> ASTSKTIEELQQEMEDLDADTTITVVQRETQKARIREQIETLRAQQMVRPSEAQLQPDVTPTQIVTFEPPRVTGFGALWIPRQQRNYMTTAYIEKIKAYVPHSNLIESGLASEAQLTSWIENTCRDYQVSMDVFMTTVLPAWIVNCIINGTSQERTNEHTWRAVIMANMEDQEVLYYPIKPIIVNAQPTLRQVMRHFGEQAVAQYMNSLQAGKPFTVKGAVTAGYANVQDAWLGIDFLRDTMQLTTKQMEVKHQIIAANVTRRKIRVFALAAPGDGDELDTERHVVDDVARGRHSLRGAQLD

Sweet potato feathery mottle virus (SPFMV) and Sweet potato mild mottle virus (SPMMV) are members of the genera Potyvirus and Ipomovirus, family Potyviridae, sharing Ipomoea batatas as common host, but transmitted, respectively, by aphids and whiteflies. A common feature for all potyvirids is the structure of virions as non-enveloped, flexible rod-shaped particles, composed of multiple copies of a unique coat protein (CP) helically arranged around the RNA genome. Here we report the generation of virus-like particles (VLPs) by transient expression of the CPs of SPFMV and SPMMV in the presence of a replicating RNA in Nicotiana benthamiana. Analysis of the purified VLPs by cryo-electron microscopy, gave structures with resolutions of 2.6 and 3.0 Å, respectively, showing a similar left-handed helical arrangement of 8.8 CP subunits per turn with the C-terminus at the inner surface and a binding pocket for the encapsidated ssRNA.

The structures of SPFMV and SPMMV were determined using single particle cryoEM with helical symmetry, at resolutions of 2.6 Å (SPFMV) and 3.0 Å (SPMMV). Each subunit is separated by helical rises of 3.97 Å and 3.98 Å and helical twists of 41.2° and 40.83°, respectively, for SPFMV and SPMMV. Coat proteins from both structures contain three domains; an N-terminal domain made up of 1–123 (SPFMV), 1–111 (SPMMV) residues, a core domain with residues 124–276 (SPFMV), 112–262 (SPMMV) and a C-terminal tail comprising 277–316 (SPFMV), 263–305 (SPMMV) residues. The cryoEM density allowed residues 91–310 (SPFMV) and residues 66–296 (SPMMV) to be modelled, identifying the major components of the three domains in each CP structure. For instance, α-helix 1, which slots in the crevice of the adjacent subunit is tilted downwards in SPMMV, compared with SPFMV and PVY N-terminal regions, with a root-mean square deviation (RMSD) of 4.7 Å. On the other hand, the predicted structure for SPMMV CP showed a flanking loop followed by helix-turn helix motif at the N-terminus, not observed in the cryoEM structure. Considering the high confidence score in this region of AlphaFold predicted structure, it is likely that this structural motif is averaged out during cryoEM 3D reconstruction due to the possible high flexibility of the N-terminal loop preceding it. The RNA segments are bound to an inner RNA binding pocket, formed by residues from the core domain and the C-terminal segment of the coat protein. In the sweet potato virus structures, these correspond to Arg 235, Ser 172 and Asp 248 (SPFMV), and Arg 262, Ser 152 and Asp 236 (SPMMV) respectively. The transition temperatures were calculated after data normalization using the first derivative of a native fraction for each sample, and the results showed that SPFMV-VLPs dissociated at 55 °C (Tm1), while the CP units unfolded at 66 °C (Tm2), whilst SPMMV-VLPs dissociated at 60 °C (Tm1), with unfolding of CP units at 69 °C (Tm2).> MKLYYKVGAASLAPHIILSEAGLPYELEAVDLKAKKTADGGDYFAVNPRGAVPALEVKPGTVITQNAAILQYIGDHSDVAA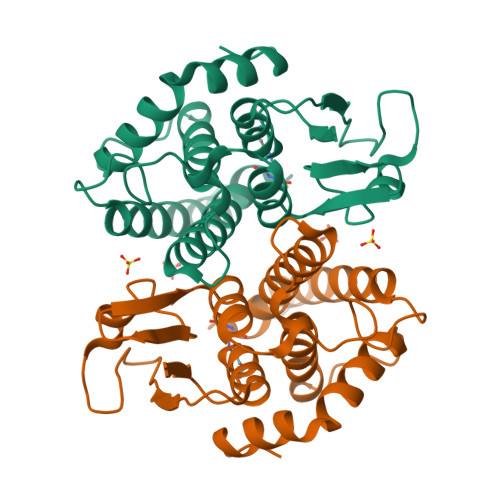FKPAYGSIERARLQEALGFCSDLHAAFSGLFAPNLSEEARAGVIANINRRLGQLEAMLSDKNAYWLGDDFTQPDAYASVIIGWGVGQKLDLSAYPKALKLRERVLARPNVQKAFKEEGLN[[(2~{R},3~{S},5~{R})-5-[5-methyl-2,4-bis(oxidanylidene)pyrimidin-1-yl]-3-oxidanyl-oxolan-2-yl]methoxy-oxidanyl-phosphoryl] 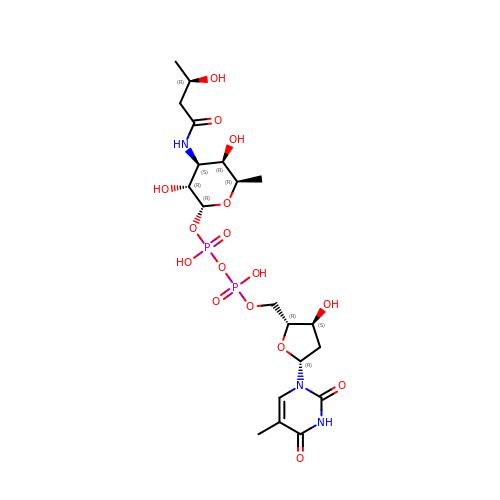[(2~{R},3~{R},4~{S},5~{R},6~{R})-6-methyl-3,5-bis(oxidanyl)-4-[[(3~{R})-3-oxidanylbutanoyl]amino]oxan-2-yl] hydrogen phosphate | C20 H33 N3 O16 P2 | SFDGKYQEVYNQBU-NKKVZDNESA-N>GHHHHHHEFDQVQYENTLKNFKIREQQFDNSWAAGFSMAALLNATKNTDTYNAHDIMRTLYPEVSEQDLPNCATFPNQMIEY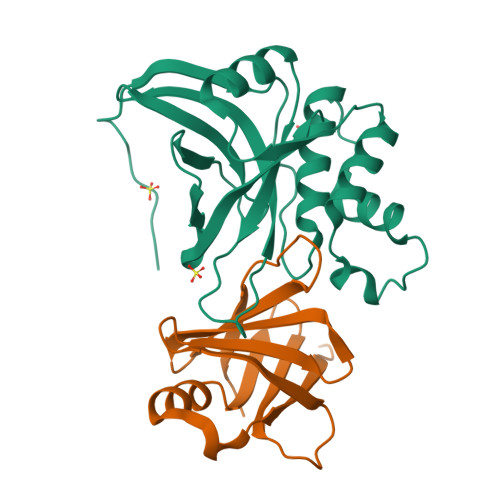GKSQGRDIHYQEGVPSYNQVDQLTKDNVGIMILAQSVSQNPNDPHLGHALAVVGNAKINDQEKLIYWNPWDTELSIQDADSSLLHLSFNRDYNWYGSMIGY[2x];>GSMYQLQFINLVYDTTKLTHLEQTNINLFIGNWSNHQLQKSICIRHGDDTSHNQYHILFIDTAHQRIKFSSFDNEEIIYILDYDDTQHILMQTSSKQGIGTSRPIVYERLV[2x]> LPQSVSRAAITAAYRRPETEAVSMLLEQARLPQPVAEQAHKLAYQLADKLRNQKNASGRAGMVQGLLQEFSLSSQEGVALMCLAEALLRIPDKATRDALIRDKISNGNWQSHIGRSPSLFVNAATWGLLFTGKLVSTHNEASLSRSLNRIIGKSGEPLIRKGVDMAMRLMGEQFVTGETIAEALANARKLEEKGFRYSYDMLGEAALTAADAQAYMVSYQQAIHAIGKASNGRGIYEGPGISIKLSALHPRYSRAQYDRVMEELYPRLKSLTLLARQYDIGININAEESDRLEISLDLLEKLCFEPELAGWNGIGFVIQAYQKRCPLVIDYLIDLATRSRRRLMIRLVKGAYWDSEIKRAQMDGLEGYPVYTRKVYTDVSYLACAKKLLAVPNLIYPQFATHNAHTLAAIYQLAGQNYYPGQYEFQCL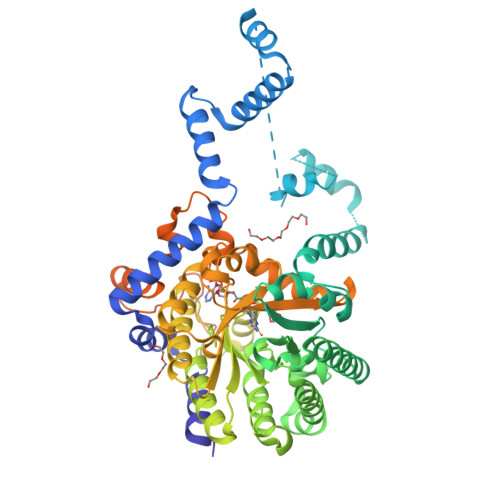HGMGEPLYEQVTGKVADGKLNRPCRIYAPVGTHETLLAYLVRRLLENGANTSFVNRIADTSLPLDELVADPVTAVEKLAQQEGQTGLPHPKIPLPRDLYGHGRDNSAGLDLANEHRLASLSSALLNSALQKWQALPMLEQPVAAGEMSPVINPAEPSSSVDKLAAALEHHHHHH2-(4-fluorophenyl)-~{N}-(4-pyridin-2-yl-1,3-thiazol-2-yl)ethanamide 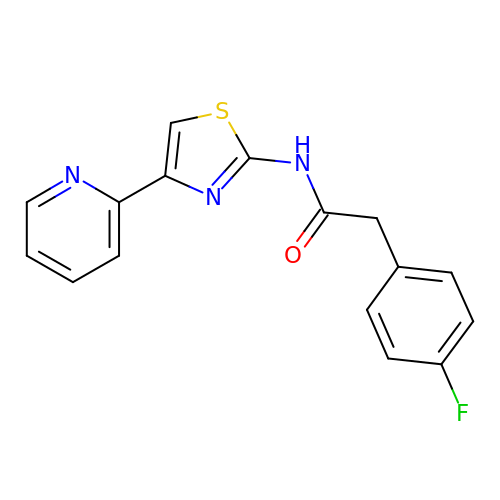| C16 H12 F N3 O S | MILLBOMBXCCZHF-UHFFFAOYSA-N> XGCGCCUGGACUUAAAGCCAUUGCACU;> CCGGCUUUAAGUUGACGAGGGCAGGGUUUAUCGAGACAUCGGCGGGUGCCCUGCGGUCUUCCUGCGACCGUUAGAGGACUGGUAAAACCACAGGCGACUGUGGCAUA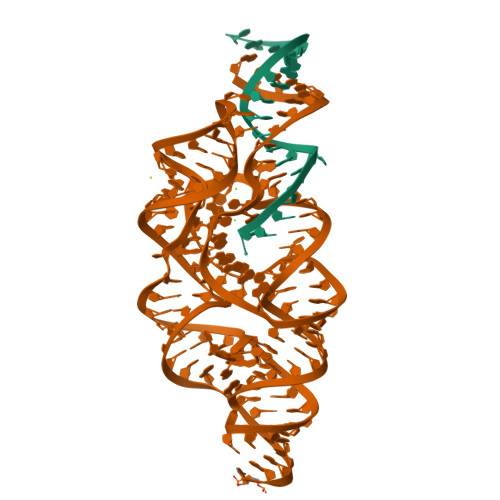GAGCAGUCCGGGCAGGAA> AVPFVEDWDLVQTLGEGAAGEVQLAVNRVTEEAVAVKIVDMKRAVDCPENIKKEICINKMLNHENVVKFYGHRREGNIQYLFLEYCSGGELFDRIEPDIGMPEPDAQRFFHQLMAGVVYLHGIGITHRDIK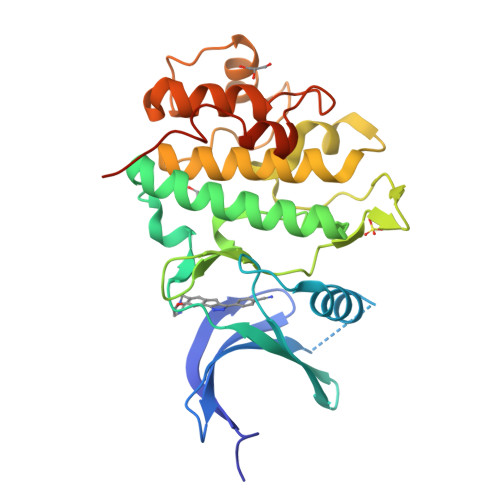PENLLLDERDNLKISDFGLATVFRYNNRERLLNKMCGTLPYVAPELLKRREFHAEPVDVWSCGIVLTAMLAGELPWDQPSDSCQEYSDWKEKKTYLNPWKKIDSAPLALLHKILVENPSARITIPDIKKDRWYNKPLKKGAKRPRVTS>[2x]GSGKMYGPGGGKYFSTTEDYDHEITGLRVSVGLLLVKSVQVKLG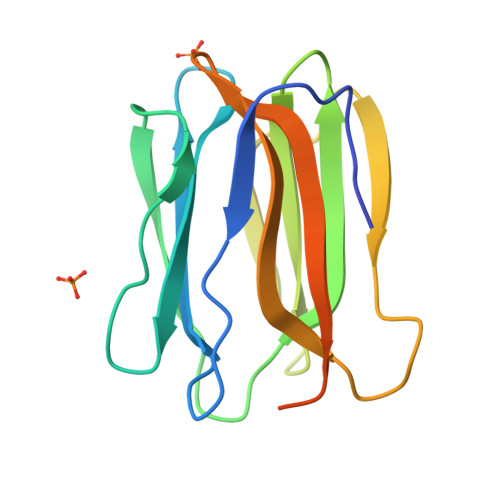DSWDVKLGALGGNTQEVTLQPGEYITKVFVAFQAFLRGMVMYTSKDRYFYFGKLDGQISSAYPSQEGQVLVGIYGQYQLLGIKSIGFEWNYPLEEPTTEPPVNLTYSANSPVGR>MAIGLPSINISFKELATTVKERSARGIIAMVLKDAKALGLNEIHEKEDIPVDLSAENKEYINLALMGNVNTPNKLLVYVIEGEADIQTALDFLETKEFNYLCMPKAVEADKTAIKNWIIKLRDIDKVKVKAVLGKVVGNHEGIINFTTEDVLVGEKKYSVDEFTSRVAGLIAGTPLSQSVTYTKLSDVVDIPKMTKVDAESRVNKGELILIKEAGAIRIARGVNSLTELTAEKGEMFQKIKIVDTLDIIHSDIRKVIIDDYIGKVTNSYDNKCLLIVAIKSYLEELEKSALIESDSTVEIDFEAQKSYLKSKGVDLSYMTLQEIKEANTGSKVFLKAKIKVLDAMEDIDLSIEI[18x];>MLKYKEILETIIEILKKNFTESIFIDDESVQGSEGSCFFVSILSVICTPVMLNTNNKDIVISIKYLPKPQSKSIRMYEISDELNKLFNRNIKVTDRKLNITKLEQSIKKEESIYVLNFTFTLNYLDSVYEEDVVYENMKEINLNLGE[6x];>MANMEARNVMSGTWGELWLDGNKVAEVKKFQAKMEFTKEDIIIAGQMGTDTKYMGYKGKGSITLYHVSSRMHKLIGEKIKRGSEPRFVAISKLNDPDSYGAERIAVKNIAFDDLTLADWEVGVKGEIEAPFTFTEYDFLDII[18x]

Here, we report the atomic structures of an engineered diffocin, a contractile syringe-like molecular machine that kills the Gram-positive bacterium Clostridioides difficile. Captured in one pre-contraction and two post-contraction states, each structure fashions six proteins in the bacteria-targeting baseplate, two proteins in the energy-storing trunk, and a collar linking the sheath with the membrane-penetrating tube. Specific attachment of baseplate tail fibers to receptors on the surface of a target bacterial cell triggers conformational changes of the neighboring baseplate, which leads to reorientation of sheath proteins and contraction of the entire sheath assembly. Since the sheath and the tube are anchored together at the opposite end by the collar, collapsing the sheath pushes the tube through the baseplate, driving it to puncture the cell wall and underlying cytoplasmic membrane.

CryoEM data processing of the post-contraction diffocin particles resolved two different substates, an apparent transitional state and a final state, which is 2 nm shorter in length. The inner tube and outer sheath are tethered together by a hexameric ring of collar protein (CD1362) at the collar-proximal end of the diffocin. The N-terminal domain of the collar subunit binds to the tube, while its C-terminal β-strand extends towards the C-terminal β-hairpin of last sheath, forming a three-β-strand handshake interaction. These interfaces are maintained during contraction, enabling the collar to function as a force transducer between sheath contraction and tube ejection. The four-layer sheath near the collar only contracts partially in the transitional state, allowing for the tube to be extended an additional 2 nm in the final state. The conformational change from the transitional state to the final state results in a 37° clockwise rotation and additional 2 nm injection of the central tube. In addition to the interface between the C-terminal β-strand of the collar and the C-terminal β-hairpin of the last sheath in the transitional state a second interface between the collar and the last sheath is observed in the final state. Lys92/97 on the N-terminal domain of the collar form salt bridges with Glu323 on the α-α corner motif of the last sheath. These interactions might provide extra mechanical stability to the junction after contraction.Three human ‘MBL-fold’ DNA repair factors, SNM1A, SNM1B (Apollo) and SNM1C (Artemis) are involved in repair of ICLs and DSBs. SNM1A–C have conserved β-CASP and metallo-β-lactamase (MBL) domains. SNM1A/SNM1B are 5′–3′ exonucleases with the unusual capacity to hydrolyse DNA substrates containing lesions, including ICLs. SNM1A has a role in replication-coupled ICL repair, functioning with the endonuclease, XPF-ERCC1, to effectively “unhook” the ICL and allow downstream processing.

The electron density maps reveal both 1 and 2 bind directly to the metal ion(s) via oxygen atoms. Two molecules of 1 were observed in the SNM1A active site, each positioned to coordinate to M1 or M2 via two oxygen ligands giving an octahedral arrangement; precedent for an MBL fold inhibitor binding mode involving two molecules comes from the observation of binding of two rhodanine derived inhibitor molecules at the active site of a true MBL. The molecule of 1 bound to the M1 site is positioned to hydrogen bond with the main chain amide of D736 and to interact with the side chains of S735, Y879 and S800. The molecule of 1 bound to the M2 site is positioned to form a potential hydrogen bond with H994 and to make a water mediated contact with Y184. The aromatic rings of both molecules of 1 stack with each other in a staggered arrangement, with the ring–ring distances between the two 1 rings being 3.2–3.5 Å. The electron density map for the SNM1A: 1 complex revealed an apparent inconsistency between the ELF reported small molecule structure and the crystallographic data. The ELF report has the methoxy group of 1 at the meta-position, however, the electron density maps clearly imply that the methoxy substituent is in the para-position for both crystallographically observed molecules of 1. The obtained structures reveal both 1 and 2 (and, likely 3) bind directly to the active site metal ion(s) of SNM1A via two oxygen atoms and likely inhibit in a competitive manner with the DNA substrate, displacing the Zn(ii) ion complexed hydrolytic water/hydroxide that, in models of the reaction mechanism, is positioned for hydrolysis of the phosphodiester bond in the DNA backbone. The three rings of 1 and 3 likely contribute to their poor solubility and hence limit their usefulness as inhibitors. It is notable, however, that the SNM1A inhibitor 1, which we subsequently used as a positive control, also inhibits both SNM1B and SNM1C with IC50 values of 1.9 μM and 0.37 μM, respectively (ESI Fig. 7†), potentially enabling efforts to target these enzymes.

> SMKKTCPFYKKIPGTGFTVDAFQYGVVEGCTAYFLTHFHSDHYAGLSKHFTFPVYCSEITGNLLKNKLHVQEQYIHPLPLDTECIVNGVKVVLLDANHCPGAVMILFYLPNGTVILHTGDFRADPSMERSLLADQKVHMLYLDTTYCSPEYTFPSQQEVIRFAINTAFEAVTLNPHALVVCGTYSIGKEKVFLAIADVLGSKVGMSQEKYKTLQCLNIPEINSLITTDMCSSLVHLLPMMQINFKGLQSHLKKCGGKYNQILAFRPTGWTHSNKFTRIADVIPQTKGNISIYGIPYSEHSSYLEMKRFVQWLKPQKIIPTVNVGTWKSRSTMEKYFREWKLEAGY> MDELGIPVYKRGFPEHLLRGYEFIIDVGTKIESVGGRHDVTKIPEMNAYDIKQESIRTALWYNPIRNDGFVLPRVLDITLRGYDERRAVVESTRHKSFHTNDQWVQWMMKDSMDAQPLKVGLDDQSRNVAHSLHNCVVKIDSKKADTMSYHVEPIEDASKGCLHTRTMMWNHLVRIETFHAAQEVAYTLKPTYDIVVHAERRDRSQPFRPGDQTLINFGRGQKVTMNHNSYDKMVEGLAHLVIRGKIPEVIRDDIASLDEICNRWIQSRHDPGEIKAYELCKILSTIGRKVLDREKEPEDEASLSIRFQEAIDNKFRQHDPERLKIFEHRNQRRDEDRFYILLMIAASDTFNTRVWWSNPYPCLRGTLIASETKLGDVYSMMRSWYDWSVRPTYTPYEKTREQEKYIYGRVNLFDFVAEPGIKIVHWEYRLNHSTREITYAQGNPCDLYPEDDDVIVTKFDDVAYGQMINEMINGGWNQEQFKMHKILKSEGNVLTIDFEKDAKLTTNEGVTMPEYFNKWIIAPMFNAKLRIKHEEIAQRQSDDPMVKRTL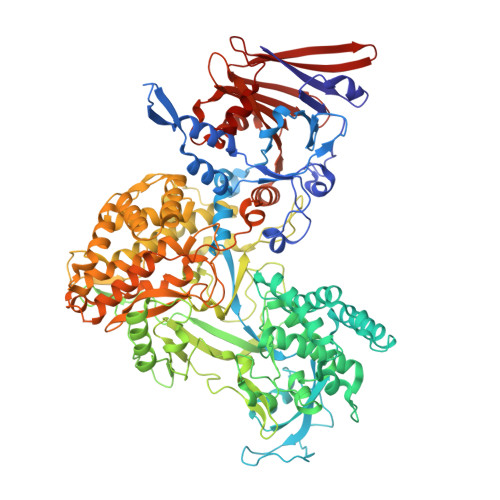SPITADPIELQRLTLARFYDIRPALRGQALSRQQAQSTYDEEISKRQDYAEILKRRGIVQIPKKPCPTVTAQYTLERYALFIISILQQHVVRDCDEEAVYEHPKADHELEIFGESIVDISQVIILAFDLIFERRRRVRDVYESRHIIARIRRMRGKERLNVIAEFFPTYGGLLNGLNSATVVQNIMYLNFLPLYFLVGDNMIYSHRQWSIPLLLYTHEVMVVPLEVGSYNDRCGLIAYLEYMVFFPSKAIRFSKLNEAQPKIAREMLKYYANTTVYDGGVNYNVVTTKQLLYETYLASLCGGISDGIVWYLPITHPNKCIVAIEVSDERVPASIRAGRIRLRFPLSARHLKGVVIIQIDEEGEFTVYSEGIVSHRVCKKNLLKYMCDIILLKFSGHVFGNDEMLTKLLNV> MSNGHV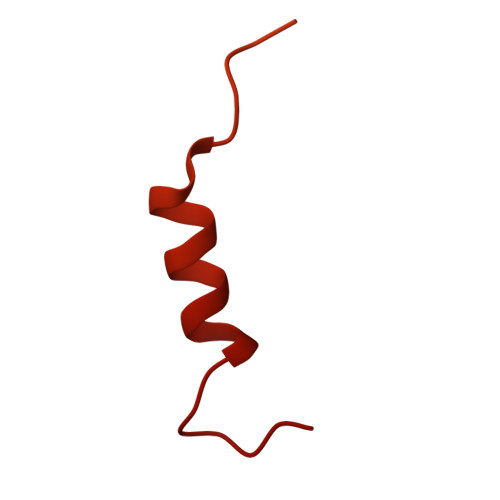KFDADESQASASAVTDRQDDVLVISKKDKEVHSSSDEESDDDDAPQEEGLHSGKSEVESQITQREEAIRLEQSQLRSKRRKQNELYAKQKKSVNETEVTDEVIAELPEELLKNIDQKDEGSTQYSSSRHVTFDKLDESDENEEALAKAIKTKKRKTLKNLRKDSVKRGKFRVQLLSTTQDSKTLPPKKESSIIRSKDRWLNRKALNKG> PGYLFSGKSNNVNEEVPTSYNQAVRRAAPAVVNVYNRSLSATQQGLAIRTLGS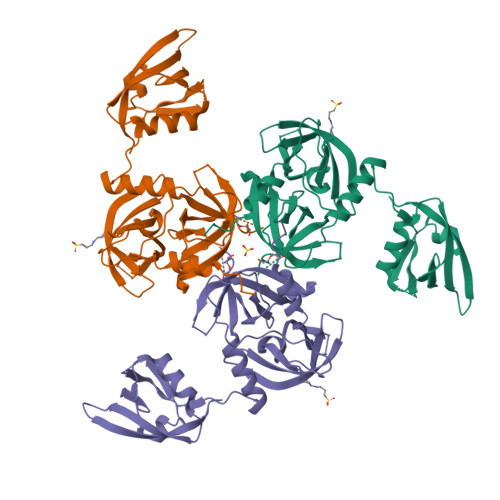GVIMSDKGYILTNKHVINDAEQIIVAMQNGRISEALLVGSDNLTDLAVLKIDATNLPVIPININRTPHIGDVVLAIGNPYNLGQTVTQGIISATGRIGLSSSGRQNFLQTDASINQGNSGGALVNTLGELMGINTLSFDKSNNGETPEGIGFAIPTALATKVMEKLIRDGRVIRGYIGITGEEYPPFNANDNGSDRVHGIKVKKVSPDGPAAQAGIHVGDIILNVNNKPATSVIETMDQVAEVRPGTTIPVLLLRNGQQIAVQITITELDQNEMLTTQAAD> MGSSHHHHHHSSGLVPRGSHMTTTISADQVNQIIYNLHHDPFEILGCHLLEEGKNTKKWVVRAYLPKAEAAWVIRPTERKEDPMNSVHHPNFFECIIETPELNHYQLKVKEGEHEKVIYDPYAFSSPYLTDEDIYLFSEGNHHRIYEKLGAHVGEINGVKGVYFAVWAPNARNVSVIGDFNNWDGREHQMRKRNYTIWELFVPEIGSGTVYKYEIKNSEGHIYEKSDPYGFYREVRPNTASIVVDIDNIYQWHDEEWLEKRRNSDPLKQPVSVYEVHLGSWLHGSSAEKMPLLNGEA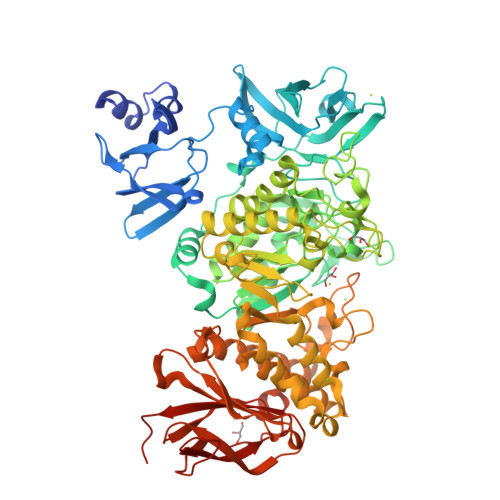DPVIVSEWNPGARFLSYYELAEKLIPYVKDMGYTHIELLPIAEHPFDGSWGYQVTGFYSPTSRFGRPEDFMYFVDKCHENGIGVILDWVPGHFPKDSHGLAYFDGTHLYEHADPRIGEHKEWGTLVFNYGRHEVRNFLVANVLFWFDKYHVDGIRVDAVASMLYRNYLRKEGEWIANEYGGDEHIEAVSFIREVNTLLFEYFPGILSIAEESTEWEKVSRPVYDGGLGFNLKWDMGWMHDMLDYFNIDPYFRQYHQNNVTFSMLYYYNENFMLALSHDEIVHGKSNMLGKMPGDEWQKYANVRALFTYMYTHPGKKTMFMSMEFGQWSEWNVNGDLEWHLLQYEPHQQLKQFFTDLNALYQQEPALYTHDFEYHGFEWIDCNDNTHSVVSFLRRSDDPNDSLVVVCNFTPQPHSHYRIGVPEAGYYVELFNSDAKQYGGSNMGNLGGKWADEWSFHNKPYSLDLCLPPLAVLILKLDPTKVPEGTTIKEIAADEEE> K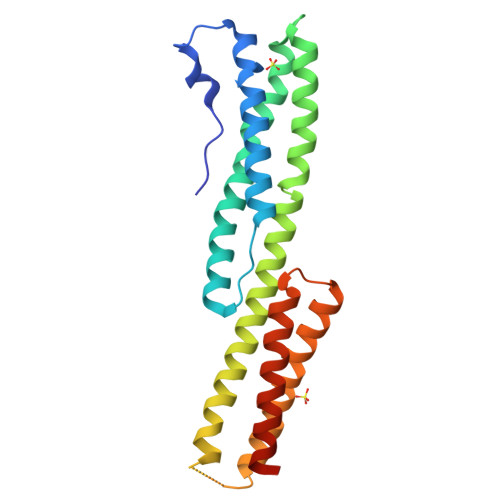LMQIRKPLLKSSLLDQNLTEEEVNMKFVQDLLNWVDEMQVQLDRTEWGSDLPSVESHLENHKNVHRAIEEFESSLKEAKISEIQMTAPLKLSYTDKLHRLESQYAKLLNTSRNQERHLDTLHNFVTRATNELIWLNEKEESEVAYDWSERNSSVARKKSYHAELMRELEQKEESIKAVQEIAEQLLLENHPARLTIEAYRAAMQTQWSWILQLCQCVEQHIQE> VIHVTKEVKEVATLSCGHNVSVEELAQTRIYWQKEKKMVLTMMSGDMNIWPEYKNRTIFDITNNLSIVILALRPSDEGTYECV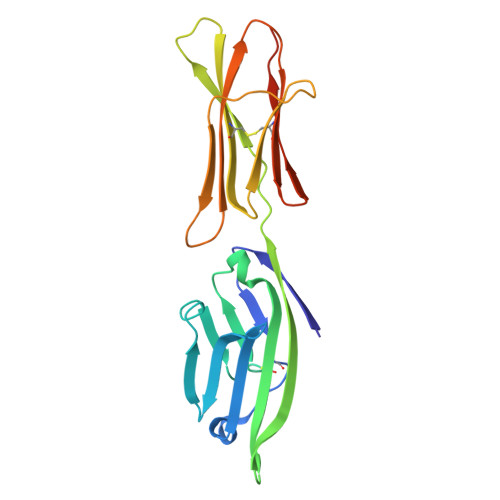VLKYEKDAFKREHLAEVTLSVKADFPTPSISDFEIPTSNIRRIICSTSGGFPEPHLSWLENGEELNAINTTVSQDPETELYAVSSKLDFNMTTNHSFMCLIKYGHLRVNQTFNWNTTKQEHFPDN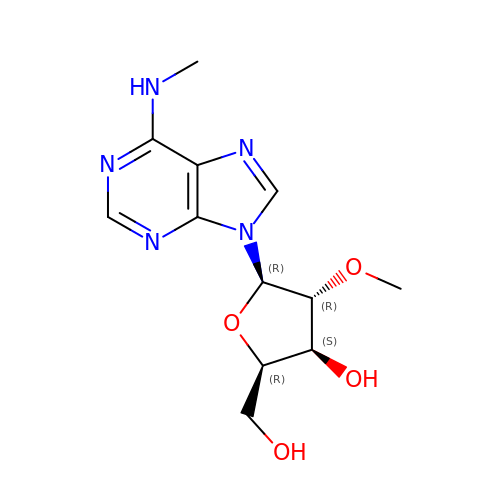(2~{R},3~{S},4~{R},5~{R})-2-(hydroxymethyl)-4-methoxy-5-[6-(methylamino)purin-9-yl]oxolan-3-ol | C12 H17 N5 O4 | GRYSXUXXBDSYRT-IQEPQDSISA-N beta-D-manno-configured 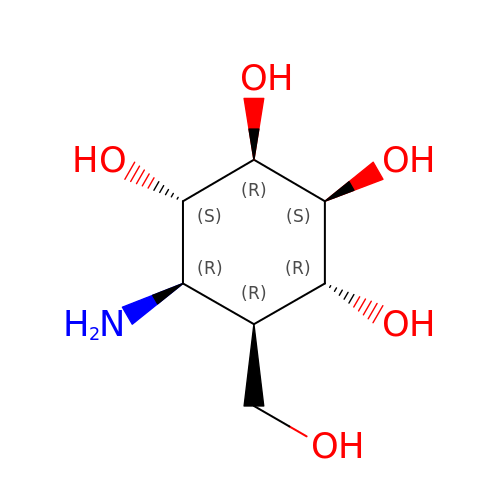cyclophellitol aziridine, reacted form | C7 H15 N O5 | SWVTZDDSAFUTKS-DOMFMGKQSA-N> MHHHHHHAMAQLGEMVTVLSIDGGGIRGIIPATILEFLEGQLQEMDNNADARLADYFDVIGGTSTGGLLTAMISTPNENNRPFAAAKEIVPFYFEHGPQIFNPSGQILGPKYDGKYLMQVLQEKLGETRVHQALTEVVISSFDIKTNKPVIFTKSNLANSPELDAKMYDISYSTAAAPTYFPPHYFVTNTSNGDEYEFNLVDGAVATVADPALLSISVATRLAQKDPAFASIRSLNYKKMLLLSLGTGTTSEFDKTYTAKEAATWTAVHWMLVIQKMTDAASSYMTDYYLSTAFQALDSKNNYLRVQENALTGTTTEMDDASEANMELLVQVGENLLKKPVSEDNPETYEEALKRFAKLLSDRKKLRANKASY

Patatin is a soluble 40 kDa non-specific plant lipase that is expressed extensively in the tubers of potatoes and other members of the nightshade family. Previously, the crystal structure of a recombinant patatin isoform, patatin-17 (pat17), derived from the tubers of heartleaf nightshade (Solanum cardiophyllum), has shown this protein to have a modified α/β hydrolase fold containing a central 6-stranded β-sheet sandwiched by 9 α-helices along with a catalytic center composed of a Ser77-Asp215 dyad. This fold and active site configuration is reminiscent of the human cytosolic phospholipase A2 family of enzymes, but it is distinct from the traditional Ser-His-Asp/Glu catalytic triads found in serine proteases and esterases such as chymotrypsin and acetylcholinesterase (AChE), respectively. Recently, interest in patatin and its homologues has been heightened by the discovery that a diverse group of mammalian lipases, termed the patatin-like phospholipase domain containing proteins (PNPLAs), encompass catalytic domains with sequence similarity to patatin.

Currently, little is known about the inhibitory potential of OP compounds such as DFP and MAFP toward patatin, beyond the fact that DFP inhibits the insecticidal ability of patatin. Consistent with this observation, we found DFP is capable of inhibiting pat17 with a 20-min IC50 of 182.1±11.1 µM. The 2.6 Å structure of pat17 co-crystallized with DFP showed an aged adduct consisting of a serine-bound DFP moiety lacking an isopropyl chain, indicating that aging had taken place. The DFP-aged structure contains a negatively charged dealkylated oxygen. This negatively charged oxygen was within hydrogen-bonding distance to the oxyanion hole (being located 2.6 Å, 2.7 Å and 3.4 Å from amide nitrogen atoms of Gly37, Gly38 and Thr78, respectively) and 5.1 Å from the Oδ2 of Asp215, which together with Ser77 comprises the catalytic dyad of patatin. Furthermore, the phosphoryl oxygen of DFP was located within hydrogen-bonding distance (2.8 Å) from the Oδ2 of Asp215. Crystals of the DFP-pat17 complex were grown in a solution with a final pH of 5.4 (measured at 4°C). Consequently, based on our structure, we propose that hydrogen bonding between this negatively charged oxygen and the protonated amide nitrogens of Gly37 and Gly38 help stabilize the negatively charged OP moiety within the active site chamber of pat17. This is expected to be similar to how the oxyanion hole helps stabilize the negatively charged tetrahedral intermediate of a native substrate during catalysis. Taken together, these observations suggest that the protonated amides in the oxyanion hole of pat17 may play a role in the aging reaction by stabilizing the emerging net negative charge on the alkoxy oxygen during the dealkylation phase of the aging process.> AELPTHYGTIIKTLRKYMKLTQSKLSERTGFSQNTISNHENGNRNIGVNEIEIY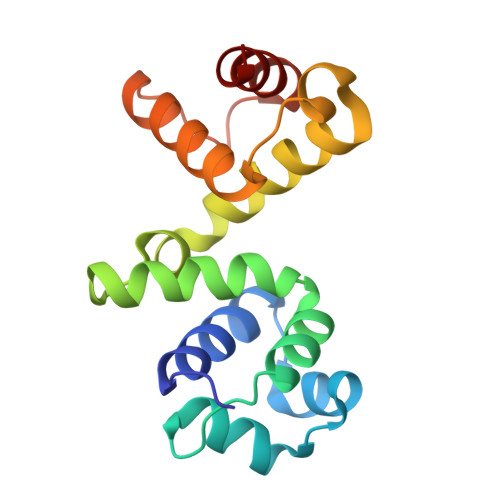GKGLGIPSYILHRISDEFKEKGYSPTLNDFGKFDKMYSYVNKAYYNDGDIYYSSYDLYDETIKLLELLKESKINVNDIDYDYVLKLYKQILST> GPANNDQDEDRINDKMKRRLAQNREAARKSRLRKKAHVQQLEESRLKLSQLEQELVRARQQGLCVRNSSDTSYLGPAGNMNSGIAAFEMEYTHWLEEQNRRVSEIRTALQAHIGDIELKMLVDSCLNHYANLFRMKADAAKADVFFLMSGMWRTSTERF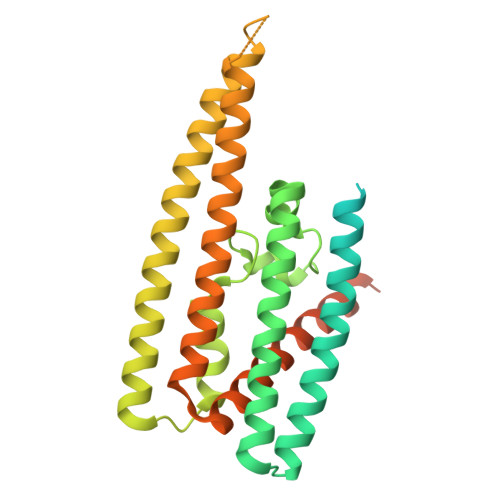FQWIGGFRPSELLNVVMPYVEPLTDQQLLEVRNLQQSSQQAEEALSQGLDKLQQGLVESIAIQIKVVESVNHGAPMASAMENLQALESFVNQADHLRQQTLQQMSKILTTRQAARGLLALGEYFHRLRALSSLWAARPREHTGGDYKDDDDKSSGYPYDVPDYA>[2x]MAHTAAERPPEETLSLWKGEQARLKARVVDRDTEAWQRDPSFSGLQKVGGVDVSFVKGDSVRACASLVVLSYPELKVVYEDSRMVGLKAPYVSGFLAFREVPFLVELVQRLQEKEPDLMPQVVLVDGNGVLHQRGFGVACHLGVLTELPCIGVAKKLLQVDGLENNALHKEKIVLLQAGGDTFPLIGSSGTVLGMALRSHDHSTKPLYVSVGHRISLEVAVRLTHHCCRFRIPEPIRQADIRSR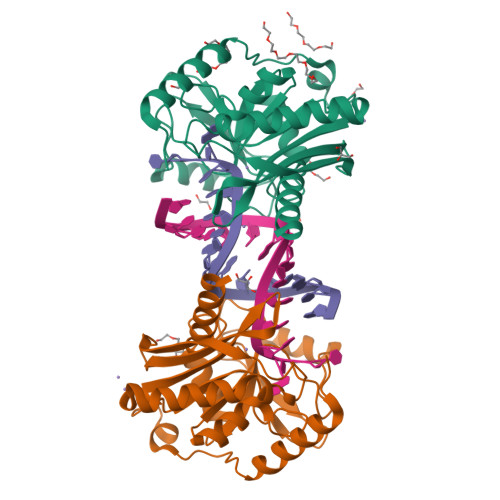EYIRRTLGQ>EVDPRLYFENRSKFIQDQKDKGINPYPHKFERTISI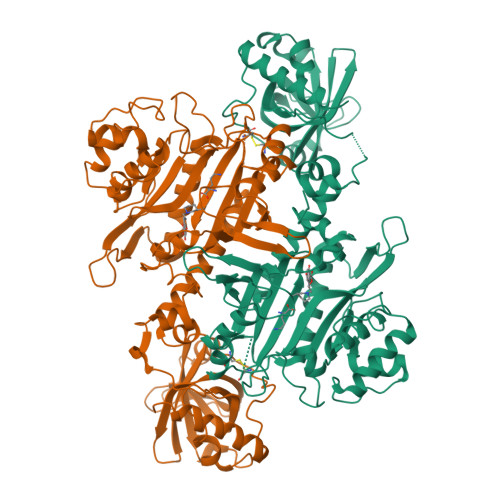PEFIEKYKDLGNGEHLEDTILNITGRIMRVSASGQKLRFFDLVGDGEKIQVLANYSFHNHEKGNFAECYDKIRRGDIVGIVGFPGKSKKGELSIFPKETILLSACLHMLPMKYGLKDTEIRYRQRYLDLLINESSRHTFVTRTKIINFLRNFLNERGFFEVETPMMNLIAGGANARPFITHHNDLDLDLYLRIATELPLKMLIVGGIDKVYEIGKVFRNEGIDNTHNPEFTSCEFYWAYADYNDLIKWSEDFFSQLVYHLFGTYKISYNKDGPENQPIEIDFTPPYPKVSIVEEIEKVTNTILEQPFDSNETIEKMINIIKEHKIELPNPPTAAKLLDQLASHFIENKYNDKPFFIVEHPQIMSPLAKYHRTKPGLTERLEMFICGKEVLNAYTELNDPFKQKECFKLQQKDREKGDTEAAQLDSAFCTSLEYGLPPTGGLGLGIDRITMFLTNKNSIKDVILFPTMRPAN[2x]>[2x]MGHHHHHHGSTTQRNAQIAMGRKKFNMDPKKGIQFLIENDLLQSSPEDVAQFLYKGEGLNKTVIGDYLGERDDFNIKVLQAFVELHEFADLNLVQALRQFLWSFRLPGEAQ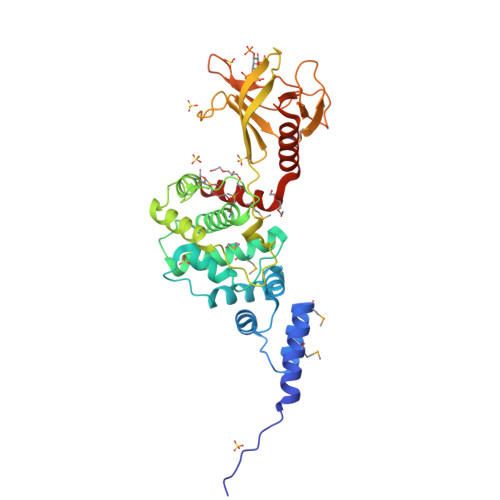KIDRMMEAFASRYCLCNPGVFQSTDTCYVLSFAIIMLNTSLHNHNVRDKPTAERFITMNRGINEGGDLPEELLRNLYESIKNEPFKIPEDDGNDLTYTFFNPDREGWLLKLGGRVKTWKRRWFILTDNCLYYFEYTTDKEPRGIIPLENLSIREVEDPRKPNCFELYNPSHKGQVIKACKTEADGRVVEGNHVVYRISAPSPEEKEEWMKSIKASISRDPFYDMLATRKRRIANKK4-[[3,5-bis(trifluoromethyl)phenyl]amino]-1,2-benzoxazol-3-one 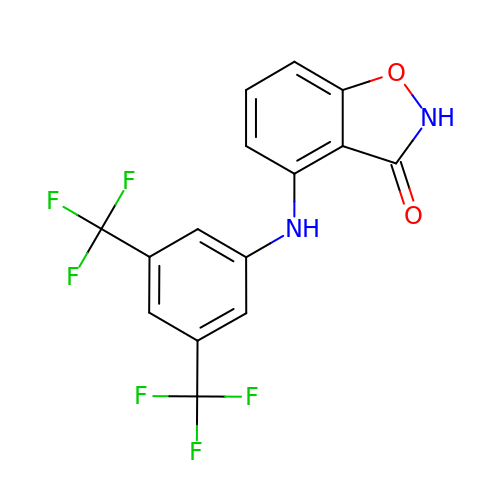| C15 H8 F6 N2 O2 | KVAIBQQTUBXORG-UHFFFAOYSA-N>[2x]MTINDSAISEQGMCEEEQVARIAWFYYHDGLTQSEISDRLGLTRLKVSRLLEKGHQSGIIRVQINSRFEGCLEYETQLRRQFSLQHVRVIPGLADADVGGRLGIGAAHMLMSLLQPQQMLAIGFGEATMNTLQRLSGFISSQQIRLVTLSGGVGSYMTGIGQLNAACSVNIIPAPLRASSADIARTLKNENCVKDVLLAAQAADVAIVGIGAVSQ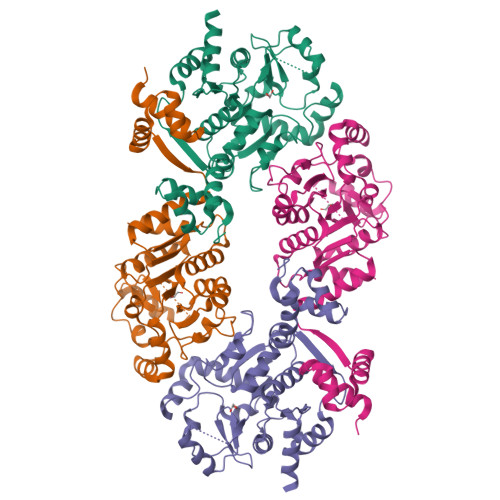QDDATIIRSGYISQGEQLMIGRKGAVGDILGYFFDAKGDVVTNIKIHNELIGLPLSALKTIPVRVGVAGGENKAEAIAAAMKGGYINALVTDQDTAAAILRSLEHHHHHH> AEILKSDAGTVDFYGQLRTELKFLEDKDPTIGSGSSRAGVDANYTVNDSLALQGKVEFAL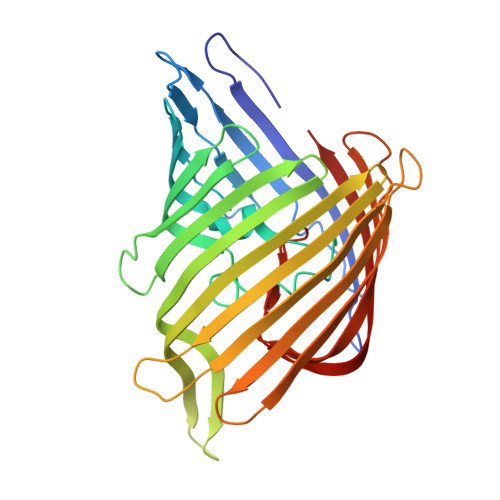KDSGDMYVRNHILGVKTNFGKFSFGKQWTTSDDVYGADYSYFFGGTGLRYGTLSDALHDSQVKYVYEADSFWVKAGYGFPEDNAKQELAELYVGATFGDLAVHAGGGQNRDKAFKVGSNTVGTTTTDIKADVTNSYFEVTGEYTIGDALIGVTYYNAELDVENNPLVIDEDAISVAGTYKVADKTKLYAGYEYVMQEANTGADEDGTLVYLGVEYKFASWARVYAEYGYGDGTTLGYTNKGSDAEVKATKVDSANNFGIGARYYW>GHMFGSINLASSLSVDAPGLQNQIDELSSFSDAPSPSVTRVLYTDKDVSARRYVKNLMALAGLTVREDAVGNIFGKWDGLEPNLPAVATGSHIDAIPYSGKYDGVVGVLGAIEAINVLKRSGFKPKRSLEIILFTSEEPTRFGISCLGSRLLAGSKELAEALKTTVVDGQNVSFIEAARSAGYAEDKD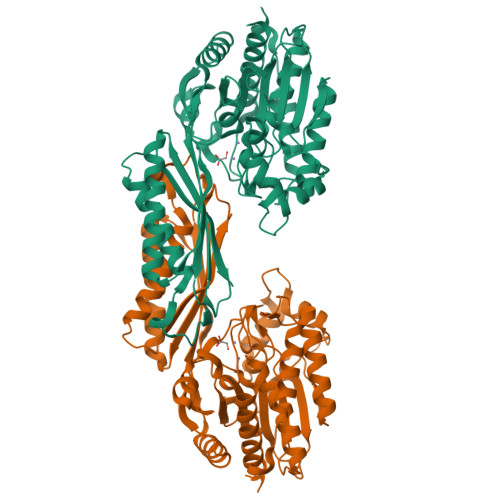DDLSSVFLKKGSYFAFLELHIEQGPILEDEGLDIGVVTAIAAPASLKVEFEGNGGHAGAVLMPYRNDAGLAAAELALAVEKHVLESESIDTVGTVGILELHPGAINSIPSKSHLEIDTRDIDEARRNTVIKKIQESANTIAKKRKVKLSEFKIVNQDPPALSDKLVIKKMAEAATELNLSHKMMISRAYHDSLFMARISPMGMIFIPCYKGYSHKPEEYSSPEDMANGVKVLSLTLAKLSLD[2x]>[2x]VSKKPSLSVQPGPIVAPEETLTLQCGSDAGYNR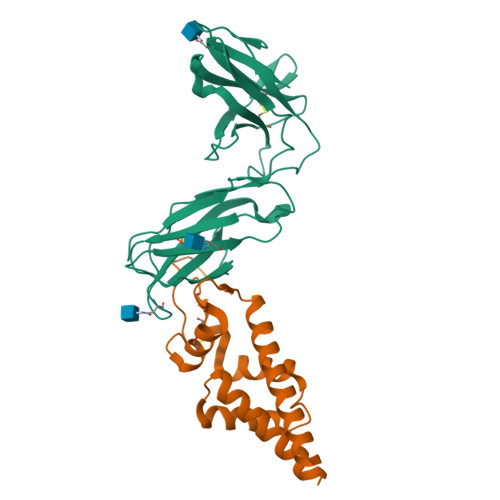FVLYKDGERDFLQLAGAQPQAGLSQANFTLGPVSRSYGGQYRCYGAHNLSSEWSAPSDPLDILIAGQFYDRVSLSVQPGPTVASGENVTLLCQSQGWMQTFLLTKEGAADDPWRLRSTYQSQKYQAEFPMGPVTSAHAGTYRCYGSQSSKPYLLTHPSDPLELVVSGGGGLEVLFQGPGGSAWSHPQFEKGGHHHHHHHH;>[2x]KELAEKAGALAGEAARIPAAIDAVIEGIKSKFSIDTLGGEALKSVIDGTNYYDASYITTAIYNKFQVSSCLPSVPFLGGPPVPGAGANKPICSAVDKLYLGSGNFLDKSSLPGSIQKDVAKIVAGAEQAAKAKAAMVASDKTLAVETAKKQ>MRIQEAIAQDKTISVIIDPSQIGSTEGKPLLSMKCNLYIHEILSRWKASLEAYHPELFLDTKKALFPLLLQLRRNQLA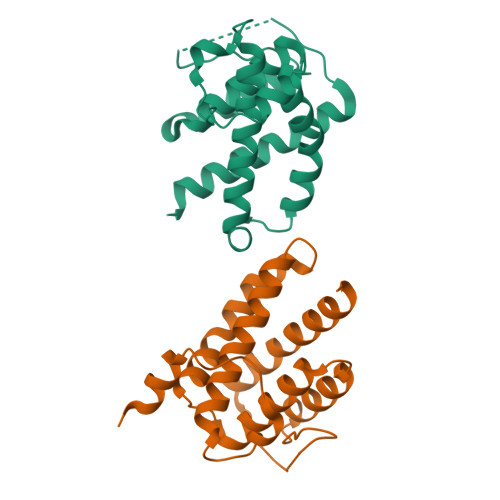PDLLISLATVLYHLQQPKEINLAVQSYMKLSIGNVAWPIGVTSVGIHARSAHSKIQGGRNAANIMIDERTRLWITSIKRLITFEEWYTSNHDSLA[2x]> MAAGGAFVSEGGGGGRSYEGGVTAFVIMTCIVAAMGGLLFGYDLGISGGVTSMEEFLTKFFPQVESQMKKAKHDTAYCKFDNQMLQLFTSSLYLAALVASFMASVITRKHGRKVSMFIGGLAFLIGALFNAFAVNVSMLIIGRLLLGVGVGFANQSTPVYLSEMAPAKIRGALNIGFQMAITIGILVANLINYGTSKMAQHGWRVSLGLAAVPAVVMVIGSFILPDTPNSMLERGKNEEAKQMLKKIRGADNVDHEFQDLIDAVEAAKKVENPWKNIMESKYRPALIFCSAIPFFQQITGINVIMFYAPVLFKTLGFGDDAALMSAVITGVVNMLSTFVSIYAVDRYGRRLLFLEGGIQMFICQLLVGSFIGARFGTSGTGTLTPATADWILAFICVYVAGFAWSWGPLGWLVPSEICPLEIRPAGQAINVSVNMFFTFLIGQFFLTMLCHMKFGLFYFFASMVAIMTVFIYFLLPETKGVPIEEMGRVWKQHWFWKKYIPEDAIIGGHDDNNTNPGLVPR

Arabidopsis thaliana STP10 is a recently characterized member of the STP family with classic STP traits. Found in growing pollen tubes, it is a proton driven symporter that displays low μM range affinity for glucose and can transport glucose, galactose and mannose. A key two-step process in apoplastic sugar import from the phloem is the breakdown of sucrose by invertases to glucose and fructose, followed by transmembrane uptake into sink cells mediated by Sugar Transport Proteins1,2. STPs display significantly higher sugar affinity compared to most other sugar Major facilitators (up to 1000× fold), and have a broad pH optimum compared to their bacterial counterparts.

The structure was determined to 2.4 Å resolution using X-ray crystallography, and the final model was refined to an Rfree of 26.8% and includes residues 21-507 (of 514 residues total). The overall structure adopts a Major Facilitator fold with 12 transmembrane helices (M1-M12) divided in two domains (N and C domain) with a quasi-twofold symmetry perpendicular to the membrane plane. STP10 is in a substrate bound outward occluded state with the N and C domains as a clamp around the central binding site. The central transmembrane binding site is located between the N and C domain and contains unambiguous density for glucose. The C domain creates a T-shaped CH-π interaction from Phe401(M10) to the main ring of glucose, while a large number of key polar interactions mediate specificity. Asn332(M10) is in contact with the hydroxyl group of glucose carbon 6 (C6) while a hydrogen bond network made through Gln295(M7), Gln296(M7), Asn301(M7), Asn433(M11), Thr437(M11), Trp410(M10) and the main chain carbonyl of Gly406(M10) and water, mediate the contact to the C1-C4 hydroxyl groups of glucose. The μM affinity of STP10 for glucose can be explained by the substrate’s interaction to residues in the N domain (Phe39 (M1b), Ile184 (M5) and in particular Leu43 (M1b)) that creates a hydrophobic interaction surface for the substrate. The Lid domain, a fully conserved feature found in all STP sequences, is a protrusion of the first extracellular loop (M1 to M2) and it is covalently linked to the C domain by a disulfide bridge (Cys77 to Cys449). Here we find the only two buried charged residues in the transmembrane region, Asp42(M1b) and Arg142(M4). The distance between Asp42 and Arg142 is ~5 Å indicating that the aspartate is in a protonated state.L-gamma-glutamyl-N-(3-ethynylphenyl)-N-hydroxy-L-glutaminylglycine | C20 H24 N4 O8 | 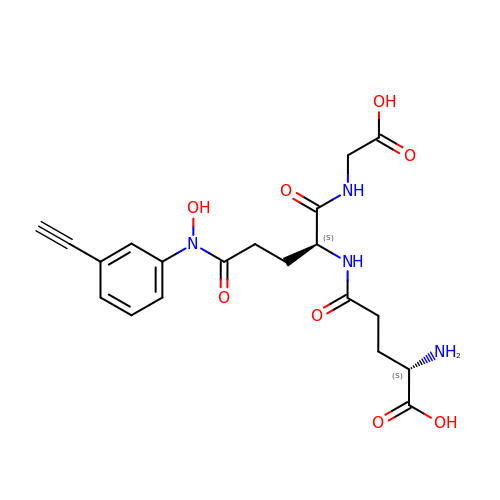DNHXPPJCZZCCCC-GJZGRUSLSA-N>MTEKKERIDVHAYLAEFDDIPGTRVFTAQRARKGYNLNQFAMSLMKAENRERFKADESAYLDEWNLTPAAKAAVLARDYNAMIDEGGNVYFLSKLFSTDGKSFQFAAGSMTGMTQEEYAQMMIDGGRSPAGVRSIKGGY[2x];>MARVTTGITSSHIPALGAAIQTGTSDNDYWGPVFKGYQPIRDWIKQPGNMPDVVILVYNDHASAFDMNIIPTFAIGCAETFKPADEGWGPRPVPDVKGHPDLAWHIAQSLILDE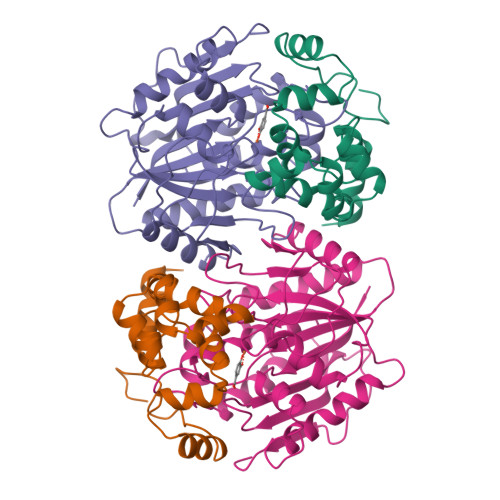FDMTIMNQMDVDHGCTVPLSMIFGEPEEWPCKVIPFPVNVVTYPPPSGKRCFALGDSIRAAVESFPEDLNVHVWGTGGMSHQLQGPRAGLINKEFDLNFIDKLISDPEELSKMPHIQYLRESGSEGVELVMWLIMRGALPEKVRDLYTFYHIPASNTALGAMILQPEETAGTPLEPRKVMSGHSLAQA[2x]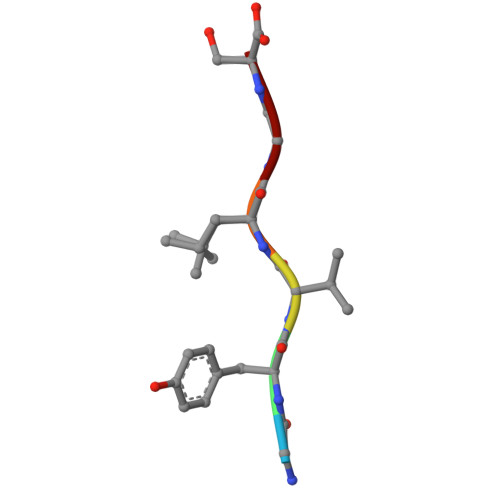>[2x]GYVLGS As a core molecular machinery in mammalian autophagy, the ULK complex is composed of a serine–threonine ULK1/2 kinase, ATG13, ATG101, and FIP200 (also named as RB1CC1), and functions as a master regulator in the initiation of autophagy under the nutrient deprivation condition by linking the upstream nutrient sensors with the downstream autophagy machines. The ULK complex initiates the autophagosome formation, and has recently been implicated in selective autophagy by interacting with autophagy receptors through its FIP200 subunit. Here, we discover that the interactions of FIP200 Claw domain with autophagy receptors CCPG1 and Optineurin can be regulated by the phosphorylation in their respective FIP200-binding regions. In all, our findings uncover a general and phosphoregulatable binding mode shared by many autophagy receptors to interact with FIP200 Claw for autophagosome biogenesis, and are valuable for further understanding the molecular mechanism of selective autophagy.

Interestingly, we also determined an apo-form crystal structure of the FIP200 Claw dimer, in which the highly positively charged LHP region of one Claw monomer is occupied by an aromatic Phe residue together with a preceding negatively charged Glu residue from the remaining sequences of the N-terminal cleaved 3C protease site of a neighboring FIP200 Claw dimer, likely due to crystal packing. Inspired by these structural observations, we inferred that an aromatic residue (Phe, Tyr, or Trp) corresponding to the I106 residue of CCPG1 FIR2 may also occupy the LHP of FIP200. Moreover, the dimerization of the FIP200 Claw domain in the FIP200 Claw/p-CCPG1 FIR2 complex is mediated by more additional polar interactions, such as the two Arg–Asp pairs (Arg1491–Asp1500) and two Arg-Glu pairs (Arg1499-Glu1494) of salt bridges, and buries a much larger surface area compared with that of the apo-form FIP200 Claw (~786 vs ~730 Å2).

>[4x]AEFSRHSEKIAIRDFQVGDLVLIILDERHDNYVLFTVSPTLYFLHSESLPALDLKPGEGASGASRRPWVLGKVMEKEYCQAKKAQNRFKVPLGTKFYRVKAVSWNKKV dimethyl 2-[[2-methyl-1-[(2-methylpropan-2-yl)oxycarbonyl]indol-3-yl]methyl]-2-prop-2-enyl-propanedioate 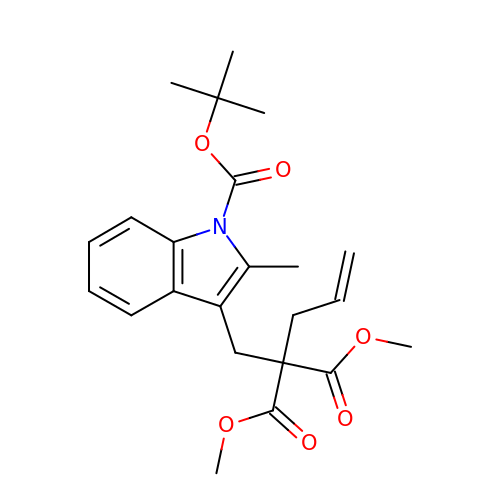| C23 H29 N O6 | VQJBZVFHBQAIGG-UHFFFAOYSA-N1,4,5,6-TETRAHYDRONICOTINAMIDE ADENINE 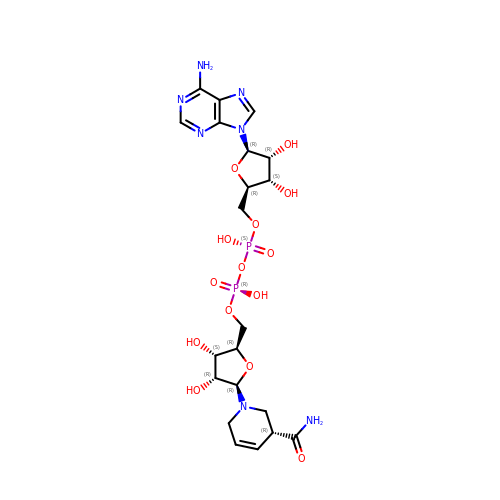DINUCLEOTIDE | C21 H31 N7 O14 P2 | GFDCQHGWOHYWLP-BFAIWXBASA-N> MSSFTKDEFDCHILDEGFTAKDILDQKINEVSSSDDKDAFYVADLGDILKKHLRWLKALPRVTPFYAVKCNDSRAIVSTLAAIGTGFDCASKTEIQLVQGLGVPAERVIYANPCKQVSQIKYAASNGVQMMTFDSEIELMKVAR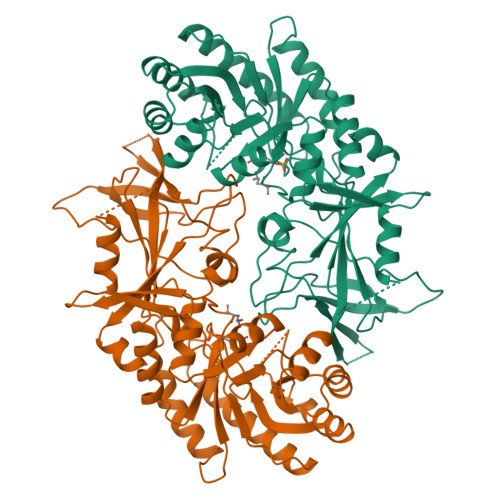AHPKAKLVLRIATDDSKAVCRLSVKFGATLKTSRLLLERAKELNIDVIGVSFHVGSGCTDPDTFVQAVSDARCVFDMATEVGFSMHLLDIGGGFPGSEDTKLKFEEITSVINPALDKYFPSDSGVRIIAEPGRYYVASAFTLAVNIIAKKTVWKEQPGSDDEDESNEQTFMYYVNDGVYGSFNCILYDHAHVKALLQKRPKPDEKYYSSSIWGPTCDGLDRIVERCNLPEMHVGDWMLFENMGAYTVAAASTFNGFQRPNIYYVMSRPMWQLMKQIQSHG>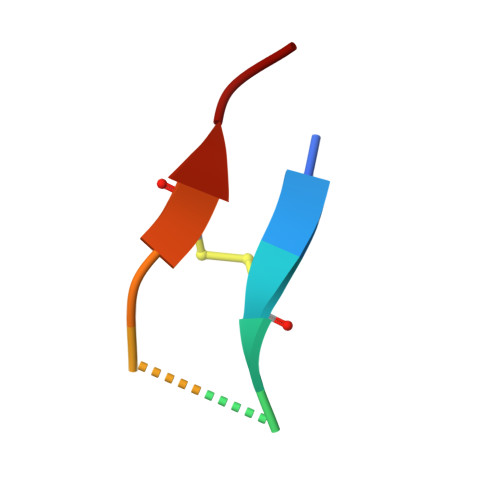 GFCQRSIPPICFPN> MHHHHHHAAGIPMNNPAIKRIGNHITKSPEDKREYRGLELANGIKVLLISDPTTDKSSAALDVHIGSLSDPPNIAGLSHFLQHMLFLGTKKYPKENEYSQFLSEHAGSSNAFTSGEHTNYYFDVSHEHLEGALDRFAQFFLSPLFDESAKDREVNAVDSEHEKNVMNDAWRLFQLEKATGNPKHPFSKFGTGNKYTLETRPNQEGIDVRQELLKFH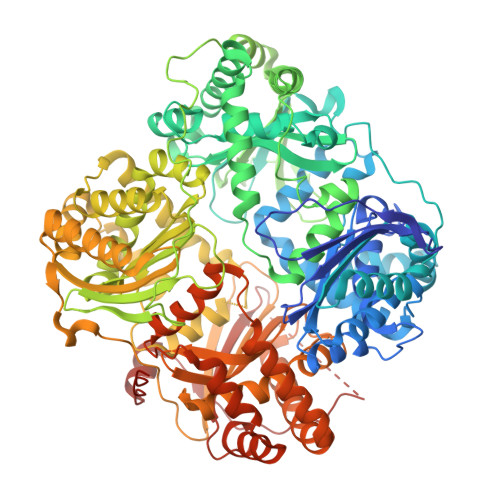SAYYSSNLMAVVVLGRESLDDLTNLVVKLFSEVENKNVPLPEFPEHPFQEEHLKQLYKIVPIKDIRNLYVTFPIPDLQKYYKSNPGHYLGHLIGHEGPGSLLSELKSKGWVNTLVGGQKEGARGFMFFIINVDLTEEGLLHVEDIILHMFQYIQKLRAEGPQEWVFQELKDLNAVAFRFKDKERPRGYTSKIAGILHYYPLEEVLTAEYLLEEFRPDLIEMVLDKLRPENVRVAIVSKSFEGKTDRTEEWYGTQYKQEAIPDEVIKKWQNADLNGKFKLPTKNEFIPTNFEILPLEKEATPYPALIKDTAMSKLWFKQDDKFFLPKANLNFEFFSPFAYVDPLHSNMAYLYLELLKDSLNEYAYAAELAGLSYDLQNTIYGMYLSVKGYNDKQPILLKKIIEKMATFEIDEKRFEIIKEAYMRSLNNFRAEQPHQHAMYYLRLLMTEVAWTKDELKEALDDVTLPRLKAFIPQLLSRLHIEALLHGNITKQAALGIMQMVEDTLIEHAHTKPLLPSQLVRYREVQLPDRGWFVYQQRNEVHNNSGIEIYYQTDMQSTSENMFLELFAQIISEPAFNTLRTKEQLGYIVFSGPRRANGIQGLRFIIQSEKPPHYLESRVEAFLITMEKSIEDMTEEAFQKHIQALAIRRLDKPKKLSAESAKYYGEIISQQYNFDRDNTEVAYLKTLTKEDIIKFYKEMLAVDAPRRHKVSVHVLAREMDSCPVVGEFPCQNDINLSQAPALPQPEVIQNMTEFKRGLPLFPLVKPHINFMAAKL>[2x]MHHHHHHRTAGPKHVLLVSEHWDLFFQT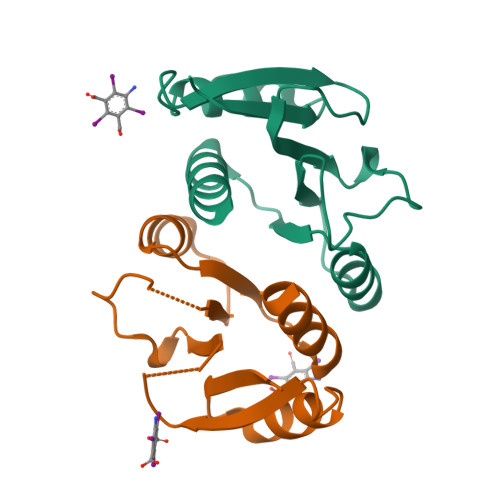KELLNPEEYRCTIGQQYKQELSADLVVCEYSLLPREIRSPKSLEGSFVLVLLDFFDEETSVDLLDRGFWYLIRPITPRILKSAISLFLSQHSL> MSNPFLRHRARVRSMRMLVADDHEANRMVLQRLLEKAGHKVLCVNGAEQVLDAMAEEDYDAVIVDLHMPGMNGLDMLKQLRVMQASGMRYTPVVVLSADVTPEAIRACEQAGARAFLAKPVVAAKLLDTLADL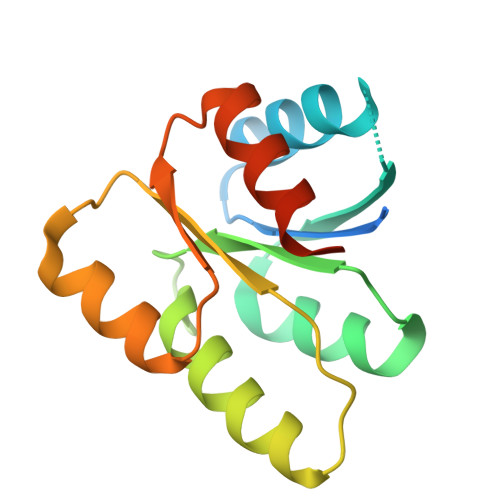AVSTRQLATP> APMNGQVCVVTGASRGIGRGIALQLCKAGATVYITGRHLDTLRVVAQEAQSLGGQCVPVV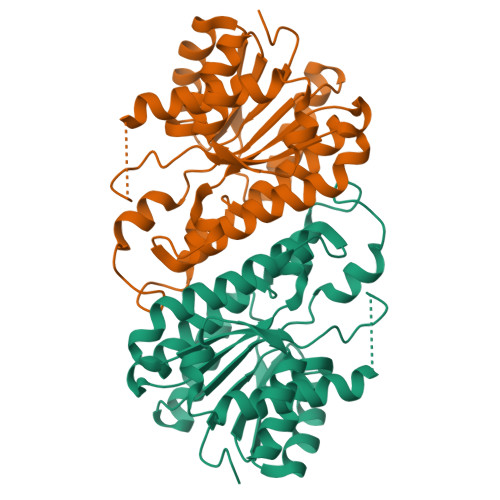CDSSQESEVRSLFEQVDREQQGRLDVLVNNAYAGVQTILNTRNKAFWETPASMWDDINNVGLRGHYFCSVYGARLMVPAGQGLIVVISSPGSLQYMFNVPYGVGKAACDKLAADCAHELRRHGVSCVSLWPGIVQTELLKEHMAKEEVLQDPVLKQFKSAFSSAETTELSGKCVVALATDPNILSLSGKVLPSCDLARRY>[4x]MTDVYILDAVRTPFGRYGGALSGIRPDDLAAHVLRALAERSPGLDPAAVDDVFFGDANGAGEDNRNVARMAALLAGWPTSVPGVTLNRLCGSGMESVIAANRAIAVGDASLAVAGGVESMSRAPWVLPKPAQGFPTGHETLYSTTLGWRMVNPAMPEQWTVSLGESTEQVAATYGISRA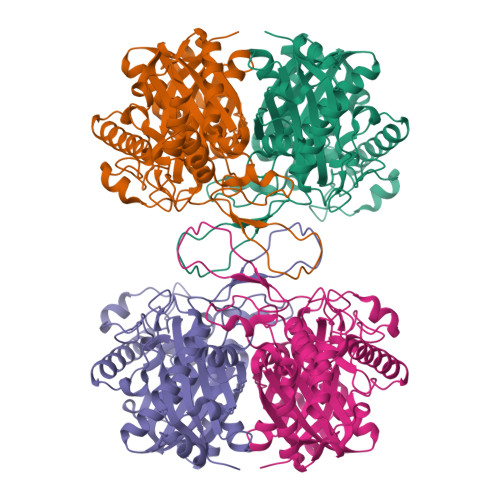EQDAFALRSHERAARAWAEGVFDAEITQIPGAELERDESIRETSAEKLAALKPAFRPDGTITAGNASPLNDGAAALLIGDAAAAERVGREPLARIVSRGVAAVDPDVFGIGPVQAAEIALRRAGIGWDDLSVVELNEAFAAQSLACLKLWPDLDPEIVNPNGGAIAIGHPLGASGARIVGTLAHELHRRGGGWGLAAICIGVGQGLAVVLHR> GSAMGSTPKDIWGRYMAKFDLAKSHGSGIYVDLGGTERVGATQHRMPTGKCPVMGKVINLGNNADFLNRISAENPQDRGLAFPDTAVAVTRNSNARNRAAAEKTEIILSPVSAADLVRWGYDGNDVANCAEYAGNIIPASDTATKYRYPFVYDAKEEMCHILFTPMQYNRGSRYCDNDGSQDEGTSSLLC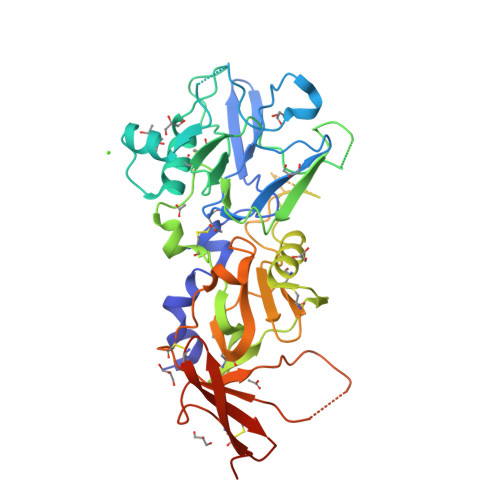MEPMKSGIDAHLYYGSSRVDKKWEENCPMYPVKDAIFGRGANGSCVAIESAFEEFTRDAEECSALMFENAAADLEIDEEADNFDELKTLSDGLRNIKASKIAQALFSPIAKAGTSAKNSKGVGMNWANYDSNTGLCRVIEETPNCLIIDAGSFAMTAVGSPLEQDAVPFPCDIVTNGYIEPRPRSRHRNTTPIFEVTTALSREALKCSKYVHEKYSESCGTYYYCSEEKPSSWAFWRNLDAAALVPR> MAYAQWVIIIIHN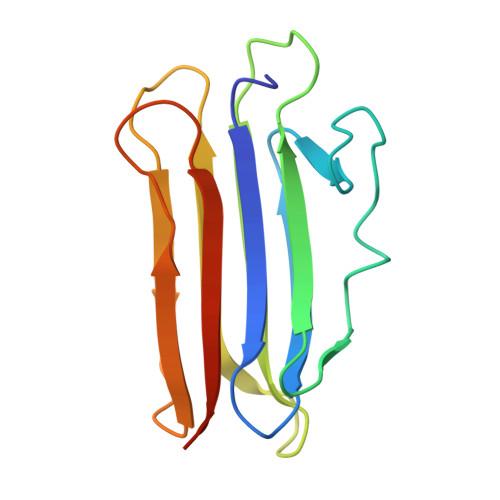VGSQDVKIKNLKASWGKLHADGDKDAEVSASNYEGKIVKPDEKLQINASGRSDAAEGTTGTFDLVDPADGDKQVRHFYWDSPWGSKTNTWTVSGSNTKWMIEYSGQNLDSGALGTITVDTLKKGENLYFQ> MAMLTKFESRSSRAKGVAFHPTQPWILTSLHNGRIQLWDYRMGTLLDRFDGHDGPVRGIAFHPTQPIFVSGGDDYKVNVWNYKSRKLLFSLCGHMDYVRVCTFHHEYPWILSCSDDQTIRIWNWQSRNCIAILTGHSHYVMCAAFHPSEDLIVSASLDQTVRVWDISGLRMKNAAPVSMSKEDQKAQAHNSISNDLFGSADAIVKFVLEGHDRGVNWCAFHPTLPLILSAGDDRLVKLWR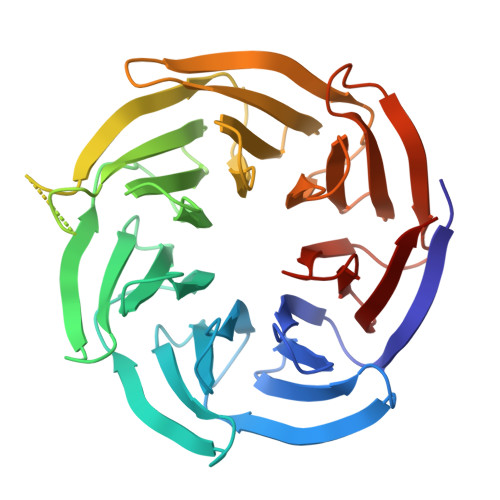MTASKAWEVDTCRGHFNNVSCCLFHPHQELILSASEDKTIRVWDLNRRTAVQTFRRANDRFWFITVHPKLNLFAAAHDSGVMVFKLE>[24x]MATINNVTDLAIAAIQWSDRQDLTQELLMLFIGNTTDRLNRLLRVRENEHFETLMAFGGGIEIPEHFVALRSITGDSLIGGRTLQYITQDIFTHYVNYNYQPQGVTYYTRLGNFWRVFPVVPDGAPFIVNY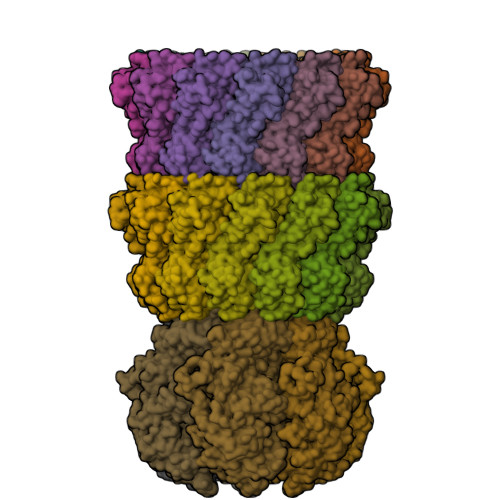WTVLPELSLANPTTWALTKYPQIYLYGVLEQIYLYTMDEARSQFWGQKLERAVMELQNEENAADFASTRLAIKDIER;>MALERQEVKNPTGIVTDIAPADLPLEKWSFGNNVRFKNGKAQKALGHTPIFDTAQAPILDMFPFIRNNIPYWLLCGEQRMYLADGTTVVDVSPGGHSASVTSRWSSGSFNGVIFANNPSNYPYVLMPQNSGFIPMPNWPANTFAKRMKSFKNFMIALNVTQNSVEMPQMVWWSTSADAGGIPVSWDPTDPTKDAGQNTLADTNGAIVDGVKLRDSFIIYKEDSVYSMRYIGGLFIFQFQQLFNDVGILGPNCAIEFDGNHFVVGHGDVYVHNGVQKQSVIDAQVRKFFFSDINPDNYQRTFVIADHVNTEMWVCYSSTRSEPGKHCDRAIIWNWKENTWSIRDLPNVLSGAYGIIDPKVSNLWDDDPNPWDTYTSVWGEGSYNPAKSSMIFSSFQDKKLFLFGNNSTFSGQNFVSTLERSDIYLGDDRMMKTVSAIIPHITGNGTCNIWVGNAQVQGSGIRWKGPYPYRIGQDYKIDTKHVGRYIALKFDFSSEGDWYFNGYTIEMAPKAGMR[6x]> VVGGTDADEGEWPWQVSLHALGQGHICGASLISPNWLVSAAHCYIDDRGFRYSDPTQWTAFLGLHDQSQRSAPG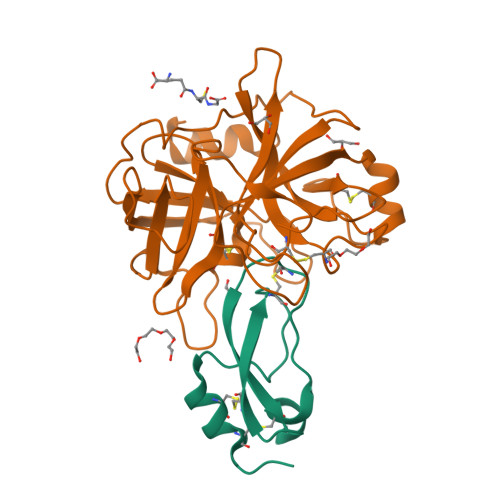VQERRLKRIISHPFFNDFTFDYDIALLELEKPAEYSSMVRPICLPDASHVFPAGKAIWVTGWGHTQYGGTGALILQKGEIRVIQQTTCENLLPQQITPRMMCVGFLSGGVDSCQGDAGGPLSSVEADGRIFQAGVVSWGDGCAQRNKPGVYTRLPLFRDWIKENTGV;> QTEDYCLASNKVGRCRGSFPRWYYDPTEQICKSFVYGGCLGNKNNYLREEECILACRGVQ> STIHQHVDESQSSLHHTEKQIQTFSTQHNNSFQELDLTNHHDVT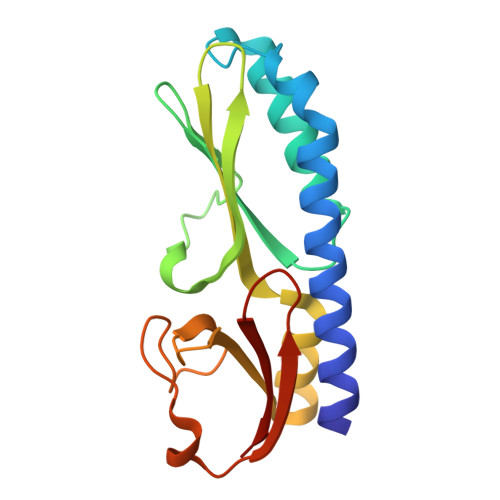ATKRELLKLIHQQPATLYYELSGPNQFITNNYEHLNTKNMYLFSTHQLKFKNSTYMLKIYMANTPRLSEIKKDNRQFALIVDQYDNILYANDDRFTIGEKYRPQQFGFMNESVKLNHADHRLIIYKDI>[2x]MAKKTPPLVFYWIPWFGSAASYGQQPYEFFESCRQKYGDVFSFMLLGKIMTVYLGPKGHEFVFNAKLSDVSAEEAYKHLTTPVFGTGVIYDCPNSRLMEQKKF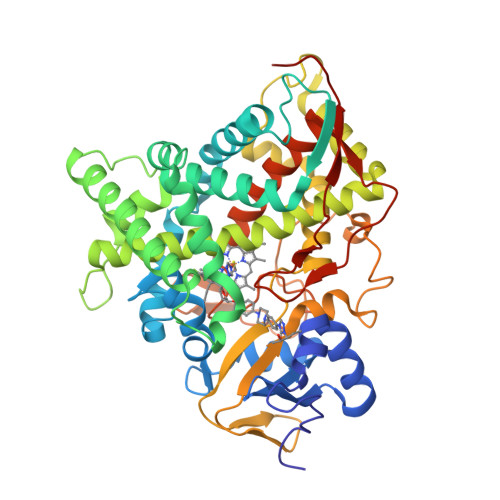AKFALTTDSFKRYVPKIREEILNYFVTDESFKLKEKTHGVANVMKTQPEITIFTASRSLFGDEMRRIFDRSFAQLYSDLDKGFTPINFVFPNLPLPHYWRRDAAQKKISATYMKEIKLRRERGDIDPNRDLIDSLLIHSTYKDGVKMTDQEIANLLIGILMGGQHTSASTSAWFLLHLGEKPHLQDVIYQEVVELLKEKGGDLNDLTYEDLQKLPSVNNTIKETLRMHMPLHSIFRKVTNPLRIPETNYIVPKGHYVLVSPGYAHTSERYFDNPEDFDPTRWDTAAAKANSVSFNSSDEVDYGFGKVSKGVSSPYLPFGGGRHRCIGEQFAYVQLGTILTTFVYNLRWTIDGYKVPDPDYSSMVVLPTEPAEIIWEKRETCMFHHHH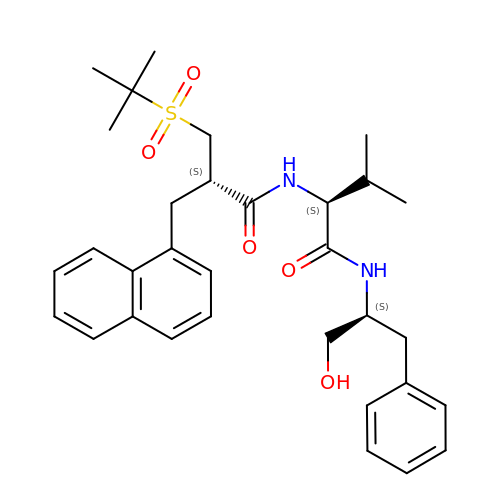[2-(2-METHYL-PROPANE-2-SULFONYLMETHYL)-3-NAPHTHALEN-1-YL-PROPIONYL-VALINYL]-PHENYLALANINOL | C32 H42 N2 O5 S | DRAZKRRTKFXIQX-XQFUHLNNSA-N Ethyl Coenzyme A | C20 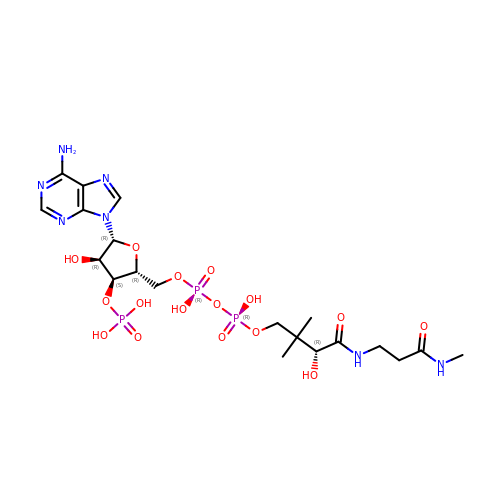H34 N7 O16 P3 | SJVFOTSCUDUYRA-BUQKYKDUSA-N>MKPKLMYQELKVPAEEPANELPMNEIEAWKAAEKKARWVLLVLILAVVGFGALMTQLFLWEYGDLHLFGPNQRPAPCYDPCEAVLVESIPEGLDFPNASTGNPSTSQAWLGLLAGAHSSLDIASFYWTLTNNDTHTQEPSAQQGEEVLRQLQTLAPKGVNVRIAVSKPSGPQPQADLQALLQSGAQVRMVDMQKLTHGVLHTKFWVVDQTHFYLGSANMDWRSLTQVKELGVVMYNCSCLARDLTKIFEAYWFLGQAGSSIPSTWPRFYDTRYNQETPMEICLNGTPALAYLASAPPPLCPSGRTPDLKALLNVVDNARSFIYVAVMNYLP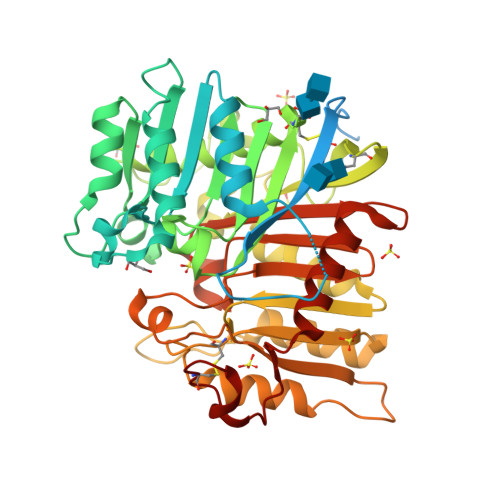TLEFSHPHRFWPAIDDGLRRATYERGVKVRLLISCWGHSEPSMRAFLLSLAALRDNHTHSDIQVKLFVVPADEAQARIPYARVNHNKYMVTERATYIGTSNWSGNYFTETAGTSLLVTQNGRGGLRSQLEAIFLRDWDSPYSHDLDTSADSVGNACRLL[2x]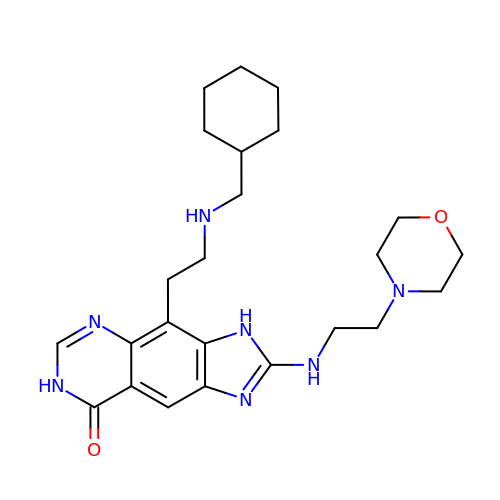4-{2-[(cyclohexylmethyl)amino]ethyl}-2-{[2-(morpholin-4-yl)ethyl]amino}-3,7-dihydro-8H-imidazo[4,5-g]quinazolin-8-one | C24 H35 N7 O2 | OAKOZMGOTCCZPS-UHFFFAOYSA-N(4~{R})-6-[(~{E})-5-(7-methoxy-3,4-dihydro-2~{H}-quinolin-1-yl)pent-1-enyl]-4-methyl-1,3,4,5-tetrahydro-1,5-benzodiazepin-2-one 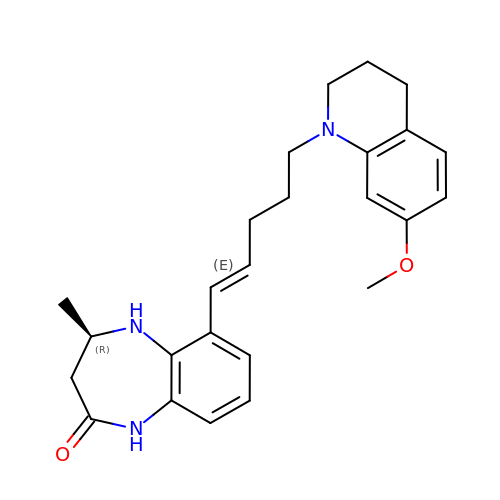| C25 H31 N3 O2 | VBTDHMQUNCGCSZ-SBLNNXNXSA-N>MTEDNIAPITSVKVVTDKCTYKDNELLTKYSYENAVVTKTASGRFDVTPTVQDYVFKLDLKKPEKLGIMLIGLGGNNGSTLVASVLANKHNVEFQTKEGVKQPNYFGSMTQCSTLKLGIDAEGNDVYAPFNSLLPMVSPNDFVVSGWDINNADLYEAMQRSQVLEYDLQQRLKAKMSLVKPLPSIYYPDFIAANQDERANNCINLDEKGNVTTRGKWTHLQRIRRDIQNFKEENALDKVIVLWTANTERYVEVSPGVNDTMENLLQSIKNDHEEIAPSTIFAAASILEGVPYINGSPQNTFVPGLVQLAEHEGTFIAGDDLKSGQTKLKSVLAQFLVDAGIKPVSIASYNHLGNNDGYNLSAPKQFRSKEISKSSVIDDIIASNDILYNDKLGKKV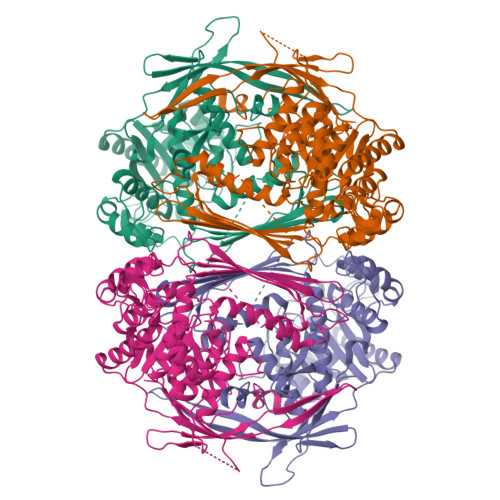DHCIVIKYMKPVGDSKVAMDEYYSELMLGGHNRISIHNVCEDSLLATPLIIDLLVMTEFCTRVSYKKVDPVKEDAGKFENFYPVLTFLSYWLKAPLTRPGFHPVNGLNKQRTALENFLRLLIGLPSQNELRFEERLL[2x]>MENTENSVDSKSIKNLEPKIIHGSESMDSGISLDNSYKMDYPEMGLCIIINNKNFHKSTGMTSRSGTDVDAANLRETFRNLKYEVRNKNDLTREEIVELMR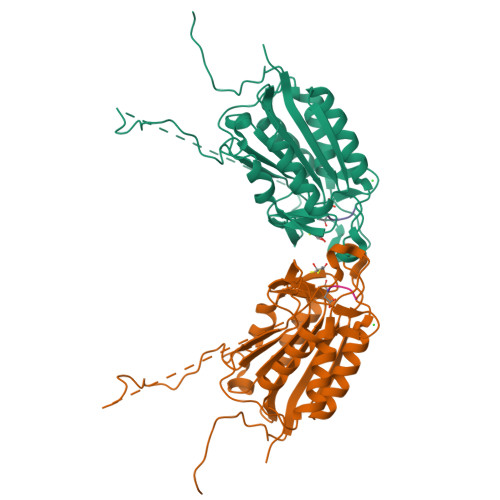DVSKEDHSKRSSFVCVLLSHGEEGIIAGTNGPVDLKKITNFFRGDRCRSLTGKPKLFIIQACRGTELDCGIETDSGVDDDMACHKIPVEADFLYAYSTAPGYYSWRNSKDGSWFIQSLCAMLKQYADKLEFMHILTRVNRKVATEFESFSFDATFHAKKQIPCIHSMLTKELYFYHL[2x]>NYMGNPWTEYMAKYDIEEVHGSGIRVDLGEDAEVAGTQYRLPSGKCPVFGKGIIIENSNTTFLTPVATGNQYLKDGGFAFPPTEPLMSPMTLDEMRHFYKDNKYVKNLDELTLCSRHAGNMIPDNDKNSNYKYPAVYDDKDKKCHILYIAAQENNGPRYCNKDESKRNSMFCFRPAKDISFQNYTYLSKNVVDNWEKVCPRKNLQNAKFGLWVDGNCEDIPHVNEFPAIDLFECNKLVFELSASDQPKQYEQHLTDYEKIKEGFKNKNASMIKSAFLPT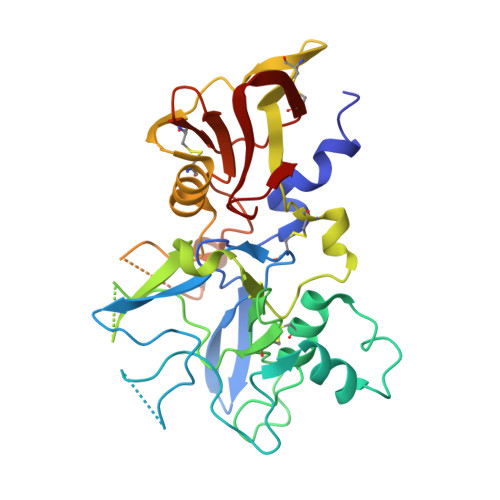GAFKADRYKSHGKGYNWGNYNTETQKCEIFNVKPTCLINNSSYIATTALSHPIEVE[2x]>[2x]MNTKYNKEFLLYLAGFVDGDGSIIAQIKPNQ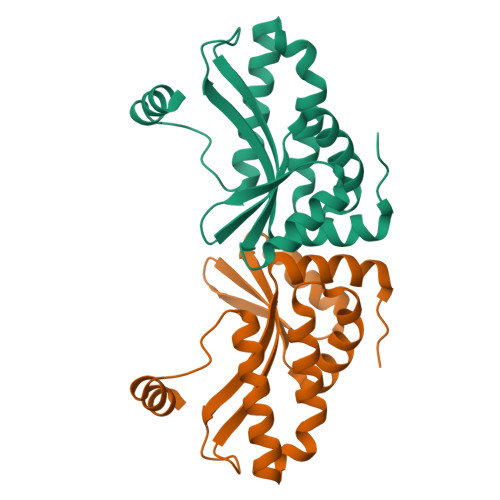SYKFKHQLSLTFQVTQKTQRRWFLDKLVDEIGVGYVRDRGSVSDYILSEIKPLHNFLTQLQPFLKLKQKQANLVLKIIEQLPSAKESPDKFLEVCTWVDQIAALNDSKTRKTTSETVRAVLDSLS> GHMASMLYLLDKSDYPKVKHLVRTKEEKSDVPLNAVINGTNVGNIYVDDPDHPKAALVDAVGTTCFLIGDASSPVFGEHLKDCIENQLKDQCLESGGSYFIATLFDKEWEKVLENAISHREYEPDYEFYHEFDKDKFNKVKSNYRSLTNEYTIKRMDKELIQNDSDDTLRSCLSDFWDSIDDFLTKGVGFCVIKDEQVISSCFTCYVDGNNHEISVETYDEEEQNKGLATKACEVYLEYCIENGITPHWSTFETNVESVNLASKLGFEYRFKLKTYEFEY

Paenibacillus larvae, the causative agent of the devastating honey-bee disease American Foulbrood, produces the cationic polyketide-peptide hybrid paenilamicin that displays antibacterial and antifungal activity. The pam gene cluster harbors a gene encoding the putative acetyl-CoA-dependent N-acetyltransferase PamZ, which belongs to the Gcn5-related N-acetyltransferase (GNAT) superfamily. We show that PamZ acts as self-resistance factor in Paenibacillus larvae by deactivation of paenilamicin. Our data unequivocally demonstrated that PamZ mono-N-acetylates the N-terminal amino group at Aga-6 position of paenilamicin and thereby abolishes its antibacterial activity.

Here, we further determined the crystal structure of PamZ:acetyl-CoA complex at 1.34 Å resolution. PamZ comprises an N-terminal domain (NTD, residues 1–128, secondary structure elements indicated by primes) and a C-terminal domain (CTD, residues 140–275), which both adopt the characteristic GNAT fold. The two tandem-GNAT domains, that may have originated from a gene duplication event, share low sequence identity (<20%) and are connected by an α-helical linker (αbridge, residues 129–139). Furthermore, the well-conserved pyrophosphate-binding loop (P-loop) of the GNAT family (R/Q-X-X-G-X-A/G)26 is only present in the CTD of PamZ (Q-N-K-G-L-A) between strand β4b and helix α3, whereas the NTD is missing this signature motif. Accordingly, there is only one acetyl-CoA molecule canonically bound in the PamZ structure, namely to the CTD. Interestingly, a major interface in PamZ is achieved by domain swapping of strand β6 (β6’), which inserts between strands β5’ and β6’ (β5 and β6) of the opposing domain and thus forms an extended, antiparallel, and strongly-twisted β-sheet throughout the enzyme. Although we did not obtain crystals of a ternary PamZ-acetyl-CoA-paenilamicin complex, the position of acetyl-CoA, the well-defined shape of the neighboring pocket and our knowledge about the substrate’s N-terminal acetylation site allows us to predict that the Glm/Aga side chain of paenilamicin very likely penetrates into this pocket. Acidic residues D25 (loop between α1’ and α2’), E122 (β6’), and E208 (β4a) are well-positioned within the pocket to accommodate and stabilize the guanidine group of Aga, as well as to tolerate the Nζ amine of Glm.> LDRADILYNIRQTSRPDVIPTQRDRPVAVSVSLKFINILEVNEITNEVDVVFWQQTTWSDRTLAWNSSHSPDQVSVPISSLWVPDLAAYNAISKPEVLTPQLARVVSDGEVLYM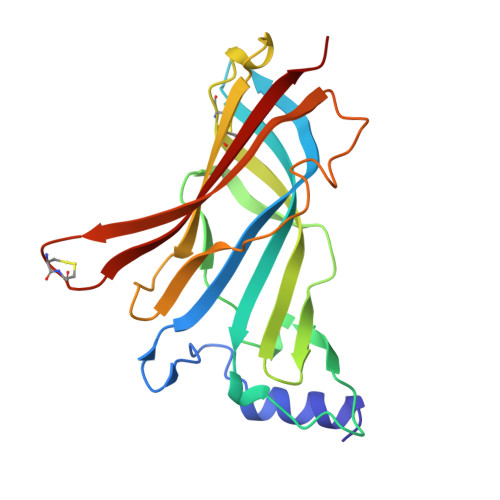PSIRQRFSCDVSGVDTESGATCRIKIGSWTHHSREISVDPTTENSDDSEYFSQYSRFEILDVTQKKNSVTYSCCPEAYEDVEVSLNFRKKG>GAMGGWAIAVHGGAGVDPTLPLERQEEAKQLLTRCLNLGISALNSNVPAIDVVELVVRELETDPLFNSGRGSALTEKGTVEMEASIMDGPKRRCGAVSGLTTVKNPISLARLVMDKSPHSYIAFSGAEDFARQQGVEVVDNEYFVTPDNVGMLKLAKEANTILFDYRIPSSAYETCGSGVESPLQMNGLPISVYAPE[2x];>[2x]TVGCVVVDREGRCAAATSTGGLMNKMTGRIGDSPLIGAGTYACDVCGVSCTGEGEAIIRGTLAREVAAVMEYKGLKLHQA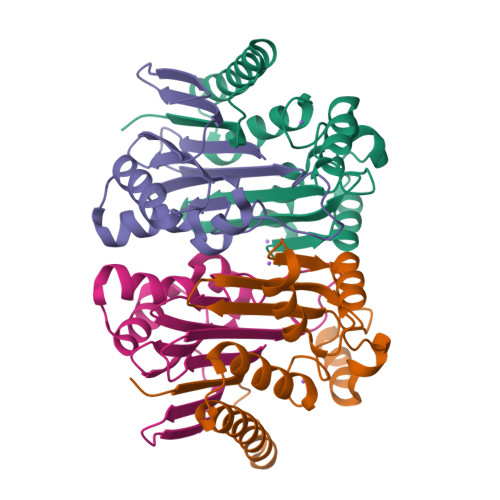VDFVIKHRLDEGKAGLIAVSNTGEVACGFNCNGMFRACATEDGFMEVAIWD> GSIAPYLVKIIDPDYEKNERTRIKAQENLRRIRRKQIAEKGDNEDGTDDPSRRRKIDDLVLNEYENQVALEVVAPEDIPVGFNDIGGLDDIIEELKETIIYPLTMPHLYKHGGALLAAPSGVLLYGPPGCGKTMLAKAVAHESGASFINLHISTLTEKWYGDSNKIVRAVFSLAKKLQPSIIFIDEIDAVLGTRRSGEHEASGMVKAEFMTLWDGLTSTNASGVPNRIVVLGATNRINDIDEAILRRMPKQFPVPLPGLEQRRRILELVLRGTKRDPDFDLDYIARVTAGMSGSDIKETCRDAAMAPMREYIRQHRASGKPLSEINPDDVRGIRTEDFFGRRGGKILSEIPPRQT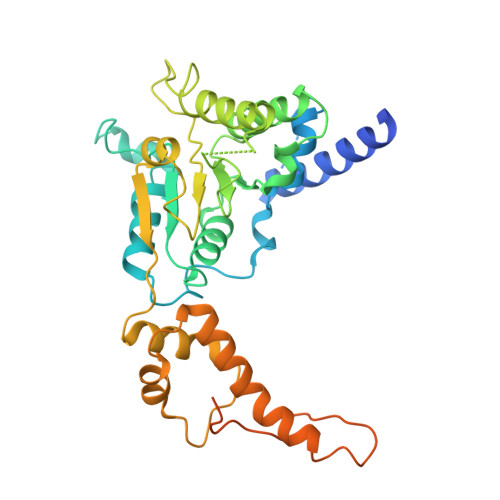GYVVQSKNSSEGGYEEVEDDDEQGTAST> PCVVGGQADTIYPAIANQMAHQMHEDAQTEASKRGLAKLRADAKQGIYKKNRKPQELSNICNITLQHSNDSRNGNNGGACTGKDGNNERFKIGTEWKIGEKVETTDTDAYIPPRRQHMCTSNLENLNVSWVTEDGKAIHSLLGDVQLAAKMDADEIIKRYKKHNTLTDPIQQKDQESICRAVRYSFADLGDIIRGRDLWEHGDQTKLQGHLQIIFGKIKEEIKKKHPGINGNDKYKGDEKNNPPYKQLREDWWEANRHQVWRAMQCELKNLKKSNGDCHYNSRGTPLDDYIPQRLRWMVEWAEWFCKMQSQEYDKLMKQCSQCMSKGGDCRKGDVNCTSCEQACEEYKKKIKKWEKQWNKIKDKYEELYLQAKIAFAGTSFGGGDRDYQQMVHFFKELQKVTGDTTLGDTTSPYSTAAGYIHQEGHVDECTEQTQFCKNRNGNTASGKEDDNYTFKDPPPKYANACKCD;> QTSVSPSKVILPRGGSVLVTCSTSCDQPKLLGIETPLPKKELLLPGNNRKVYELSNVQEDSQPMCYSNCPDGQSTAKTFLTVYWTPERVELAPLPSWQPVGKNLTLRCQVEGGAPRANLTVVLLRGEKELKREPAVGEPAEVTTTVLVRRDHHGANFSCRTELDLRPQGLELFEN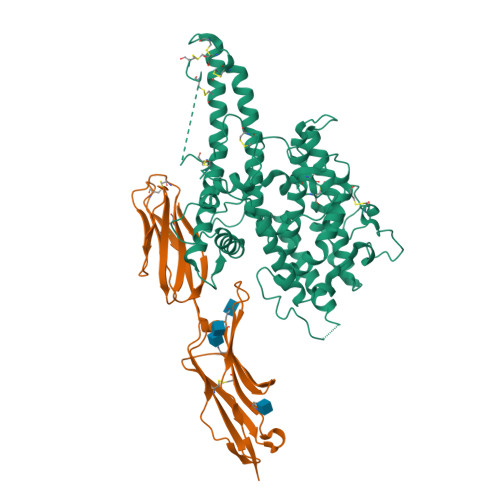TSAPYQLQTFG> GKPQYMVLVPSLLHTETTEKGCVLLSYLNETVTVSASLESVRGNRSLFTDLEAENDVLHCVAFAVPKSSSNEEVMFLTVQVKGPTQEFKKRTTVMVKNEDSLVFVQTDKSIYKPGQTVKFRVVSMDENFHPLNELIPLVYIQDPKGNRIAQWQSFQLEGGLKQFSFPLSSEPFQGSYKVVVQKKSGGRTEHPFTVEEFVLPKFEVQVTVPKIITILEEEMNVSVCGLYTYGKPVPGHVTVSICRKYSDASDCHGEDSQAFCEKFSGQLNSHGCFYQQVKTKVFQLKRKEYEMKLHTEAQIQEEGTVVELTGRQSSEITRTITKLSFVKVDSHFRQGIPFFGQVRLVDGKGVPIPNKVIFIRGNEANYYSNATTDEHGLVQFSINTTNVMGTSLTVRVNYKDRSPCYGYQWVSEEHEEAHHTAYLVFSPSKSFVHLEPMSHELPCGHTQTVQAHYILNGGTLLGLKKLSFYYLIMAKGGIVRTGTHGLLVKQEDMKGHFSISIPVKSDIAPVARLLIYAVLPTGDVIGDSAKYDVENCLANKVDLSFSPSQSLPASHAHLRVTAAPQSVCALRAVDQSVLLMKPDAELSASSVYNLLPEKDLTGFPGPLNDQDNEDCINRHNVYINGITYTPVSSTNEKDMYSFLEDMGLKAFTNSKIRKPKMCPQLQQYEMHGPEGLRVGFYESDVMGRGHARLVHVEEPHTETVRKYF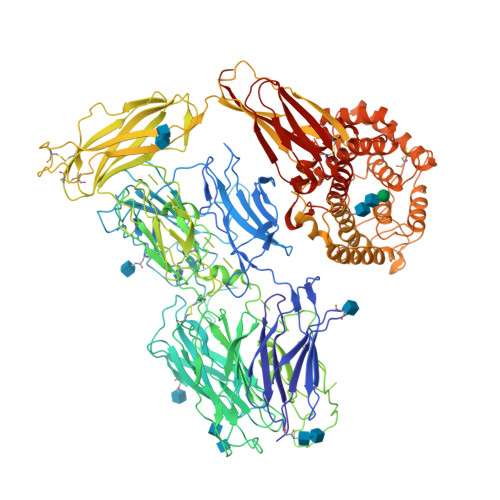PETWIWDLVVVNSAGVAEVGVTVPDTITEWKAGAFCLSEDAGLGISSTASLRAFQPFFVELTMPYSVIRGEAFTLKATVLNYLPKCIRVSVQLEASPAFLAVPVEKEQAPHCICANGRQTVSWAVTPKSLGNVNFTVSAEALESQELCGTEVPSVPEHGRKDTVIKPLLVEPEGLEKETTFNSLLCPSGGEVSEELSLKLPPNVVEESARASVSVLGDILGSAMQNTQNLLQMPYGCGEQNMVLFAPNIYVLDYLNETQQLTPEIKSKAIGYLNTGYQRQLNYKHYDGSYSTFGERYGRNQGNTWLTAFVLKTFAQARAYIFIDEAHITQALIWLSQRQKDNGCFRSSGSLLNNAIKGGVEDEVTLSAYITIALLEIPLTVTHPVVRNALFCLESAWKTAQEGDHGSHVYTKALLAYAFALAGNQDKRKEVLKSLNEEAVKKDNSVHWERPQKPKAPVGHFYEPQAPSAEVEMTSYVLLAYLTAQPAPTSEDLTSATNIVKWITKQQNAQGGFSSTQDTVVALHALSKYGAATFTRTGKAAQVTIQSSGTFSSKFQVDNNNRLLLQQVSLPELPGEYSMKVTGEGCVYLQTSLKYNILPE>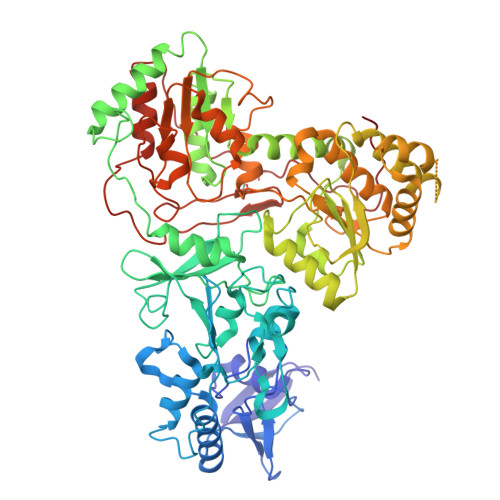 MKEITLTIDGKVCKGVQGDTILDVANKNDVYIPTLCYQKGLTPIGACRMCVVQLEGNPKMLPSCTTPAQDGMVVVTKNEKLKDYRRQILELLFAGRNHFCMYCSQSGDCELQRLAIEHEMDSVRFPYLYEDFEVDATDPNLMMDHNRCVLCQRCIRTCSEIVGAHTLDLERRGWQAKVIADLGKRLRESDTCVNCGACAQSCPTGTITIREFAYRGRRSECDAVVESVCPLCAVGCKIKTYVRTGSIVRVEGTGVEEPDGGQLCHMGRWWLPESTERERVTVPLIREGASYREATWEEALALASAEFKKAYDQEKAGAILSSLCTDEELTLFSALFRNALKMKHIDTFDGDIIRGFFKGFMPFREQGVRPFTAAHHILDSDLIITMFADPQKEAPVVASYIRVACLHRNAKLMNLSYGPSPFPGLVDLDIRLPEGQAVPKALSNLAEIIGKISLGPSDMASFGEFEAGAGKALSSYRESIEESARAMGLDPKIAEEVALMLISARRPIFIIGGRATKSHELVTAACNLAVASKAFFEDGLGVVPLLVSANSLGARNTVVSENPWLGRERRDFLYVFSTAMVPEEEEILAAISATRFVVVQTPFKVRPLVNLADILLPAPAWYERSGHFCTIEGERRKLNTIVPPKGEIKSLHYVMDEFAKKLGVKLERPEVSPCEEIFKSQLRASEARIVTL>[2x]GSMAPAMEYSTQNGQGEGKKRASVLAIGTTNPEHFILQEDYPDFYFRNTNSEHMTELKEKFKRICVKSHIRKRHFYLTEEILKENQGIATYGAGSLDARQRILETEVPKLGQEAALKAIAEWGQPISKITHVVFATTSGFMMPGADYVITRLLGLNRTVRRVMLYNQGCFAGGTALRVAKDLAENNEGARVLVVCAENTAMTFHAPNESHLDVIVGQAMFSDGAAALIIGACPDVASGERAVFNILSASQTIVPGSDGAITAHFYEMGMSYFLKEDVIPLFRDNIAAVMEEAFSPLGVSDWNSLFYSIHPGGRGIIDGVAGNLGIKDENLVATRHVLGEYGNMGSACVMFILDELRKSSKVNGKPTTGDGKEFGCLIGLGPGLTVEAVVLQSVPILQ

Type III PKS catalysis involves the loading of a CoA-tethered substrate onto an active-site cysteine followed by chain elongation via iterative decarboxylative Claisen condensations of malonyl-CoA. Linear poly­ketide intermediates undergo a terminal intramolecular cyclization reaction to produce the final cyclic polyketide product. The five-layered αβαβα topology of secondary-structural elements of each monomer is consistent with the ‘thiolase fold’ originally observed in thiolase and present in all known structures of type III PKSs.

In contrast to BIS, benzophenone synthase (BPS) generates the core chemical scaffolds of xanthones, guttiferones and sampsoniones that are prominently found in the closely related Hypericaceae and Clusiaceae families. For comparative purposes, we obtained a synthetic gene derived from the gene sequence of H. androsaemum BPS (HaBPS). Similar to previous reports, HaBPS produced 2,4,6-trihydroxybenzophenone (phlorobenzophenone) when incubated with benzoyl-CoA. Additionally, unlike MdBIS1 and MdBIS3, 4-hydroxycoumarin was not detected when HaBPS was incubated with salicoyl-CoA as a starter substrate. The crystallographic models of HaBPS and MdBIS3 contained 772 out of 790 residues and 757 out of 776 residues, respectively. A significant change in the HaBPS cavity arises from the small-to-large replacement of Leu263 in MdCHS2 with Met267 in HaBPS. Similarly, the side chain of Met267 of HaBPS replaces Leu263 of CHS and blocks access to the coumaroyl-binding area of the CHS cavity. Similarly, the side chains of Thr135 and Glu195 and the main-chain atoms of Gly166, Gly342 and Ser343 line the sides of this novel pocket in HaBPS. Mutagenesis of Thr135 in HaBPS to Leu resulted in a reduction in chain-elongation steps from three to two and a shift in the terminal cyclization mechanism from Claisen to lactonization. Presumably, a similar water-mediated hydrogen bond stabilizes Tyr269 of HaBPS; however, the lower resolution of the diffraction data for the HaBPS crystals prevented the analysis of waters. However, higher resolution structures of BPS are needed for comparisons of subtle changes in backbone, side chain and ordered waters between BPS and BIS.>MSISISYSTTYSGWTVADYLADWSAYFGDVNHRPGQVVDGSNTGGFNPGPFDGSQYALKSTASDAAFIAGGDLHYTLFSNPSHTLWGKLDSIALGDTLTGGASSGGYALDSQEVSFSNLGLDSPIAQGRDGTVHKVVYGLMSGDSSALQGQIDALLKAVDPSLSINSTFDQLAAA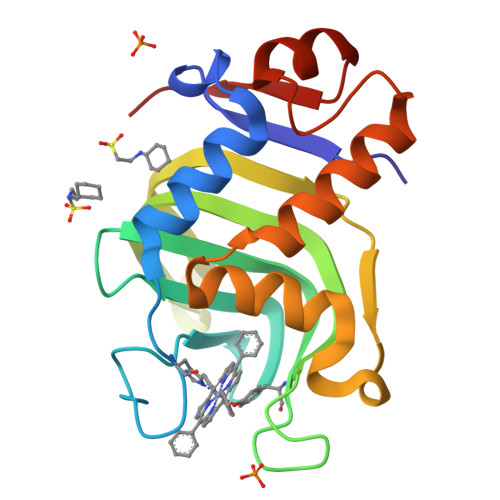GVAHATPAA[3x]> MAQFDTEYQRLEASYSDSPPGEEDLLVHVAEGSKSPWHHIENLDLFFSRVYNLHQKNGFTCMLIGEIFELMQFLFVVAFTTFLVSCVDYDILFANKMVNHSLHPTE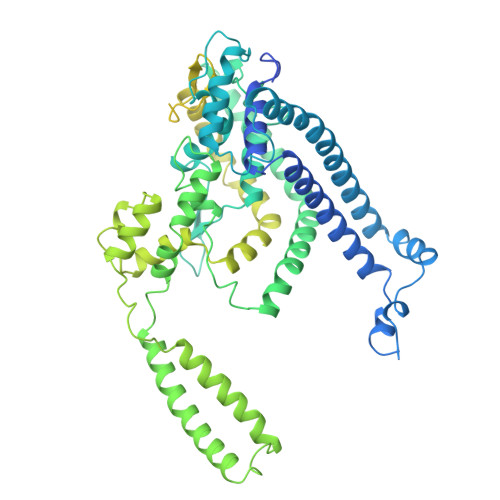PVKVTLPDAFLPAQVCSARIQENGSLITILVIAGVFWIHRLIKFIYNICCYWEIHSFYLHALRIPMSALPYCTWQEVQARIVQTQKEHQICIHKRELTELDIYHRILRFQNYMVALVNKSLLPLRFRLPGLGEAVFFTRGLKYNFELILFWGPGSLFLNEWSLKAEYKRGGQRLELAQRLSNRILWIGIANFLLCPLILIWQILYAFFSYAEVLKREPGALGARCWSLYGRCYLRHFNELEHELQSRLNRGYKPASKYMNCFLSPLLTLLAKNGAFFAGSILAVLIALTIYDEDVLAVEHVLTTVTLLGVTVTVCRSFIPDQHMVFCPEQLLRVILAHIHYMPDHWQGNAHRSQTRDEFAQLFQYKAVFILEELLSPIVTPLILIFCLRPRALEIIDFFRNFTVEVVGVGDTCSFAQMDVRQHGHPQWLSAGQTEASVYQQAEDGKTELSLMHFAITNPGWQPPRESTAFLGFLKEQVQRDGAAASLAQGGLLPENALFTSIQSLQSESEPLSLIANVVAGSSCRGPPLPRDLQGSRHRAEVASALRSFSPLQPGQAPTGRAHSTMTGSGVDARTASSGSSVWEGQLQSLVLSEYASTEMSLHALYMHQLHKQQAQAEPERHVWHRRESDESGESAPDEGGEGARAPQSIPRSASYPCAAPRPGAPETTALHGGFQRRYGGITDPGTVPRVPSHFSRLPLGGWAEDGQSASRHPEPVPEEGSEDELPPQVHKV> TDKEYISEEVQKAIDDSVKQVFGIKDDSSQVTITYNKDKVNLWTQQIIDYTIRGLNKLGKHFKY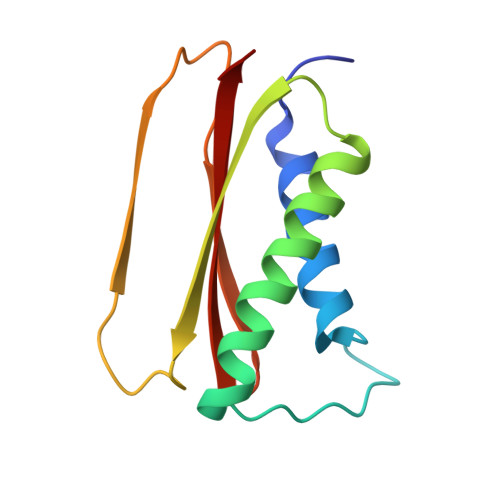CVTAILQQTNHAGISVQITAYQDTATDGSLIQCYEINDIYAIVSVFAMAV5-(phenylethynyl)pyridine-3-carboxylic acid | C14 H9 N O2 | 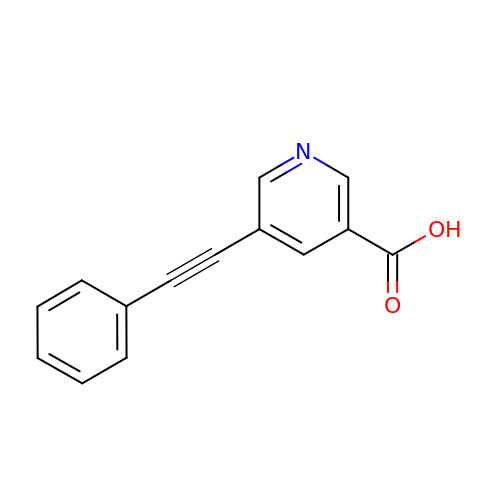DXJZBANECHYHRT-UHFFFAOYSA-N(2R)-3-{[(S)-hydroxy{[(1S,2R,3R,4S,5S,6S)-2,3,6-trihydroxy-4,5-bis(phosphonooxy)cyclohexyl]oxy}phosphoryl]oxy}propane-1,2-diyl 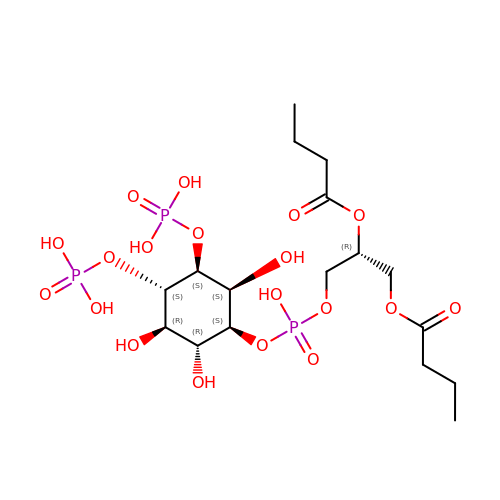dibutanoate | C17 H33 O19 P3 | DHAFWWKSHUBGAH-DXOPXGNRSA-N> XCRATK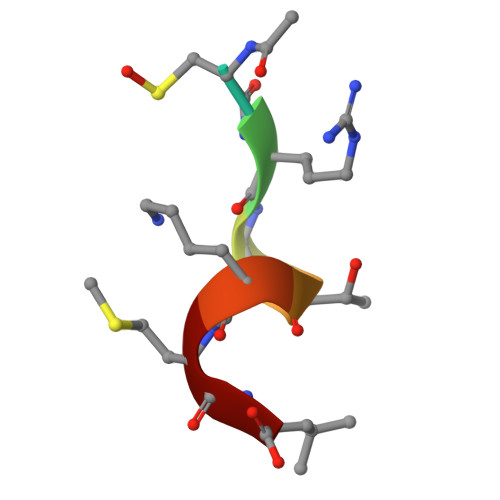ML> GPHMSSERVLSYAPAFKSFLDTSFFQELSRLKLDVLKLDSTCQPLTVNLDLHNIPKSADQVPLFLTNRSFEKHNNKRTNEVPLQGSIFNFNVLDEFKNLDKQLFLHQRALECWEDGIKDINKCVSFVIISFADLKKYRFYYWLGVPCFQRPSSTVLHVRPEPSLKGLFSKCQKWFDVNYSKWVCILDADDEIVNYDKCIIRKTKVLAIRDTSTMENVPSALTKNFLSVLQYDVPDLIDFKLLIIRQNEGSFALNATFASIDPQSSSSNPDMKVSGWERNVQGKLAPRVVDLSSLLDPLKIADQSVDLNLKLMKWRILPDLNLDIIKNTKVLLLGAGTLGCYVSRALIAWGVRKITFVDNGTVSYSNPVRQALYNFEDCGKPKAELAAASLKRIFPLMDATGVKLSIPMIGHKLVNEEAQHKDFDRLRALIKEHDIIFLLVDSRESRWLPSLLSNIENKTVINAALGFDSYLVMRHGNRDEQSSKQLGCYFCHDVVAPTDSLTDRTLDQMCTVTRPGVAMMASSLAVELMTSLLQTKYSGSETTVLGDIPHQIRGFLHNFSILKLETPAYEHCPACSPKVIEAFTDLGWEFVK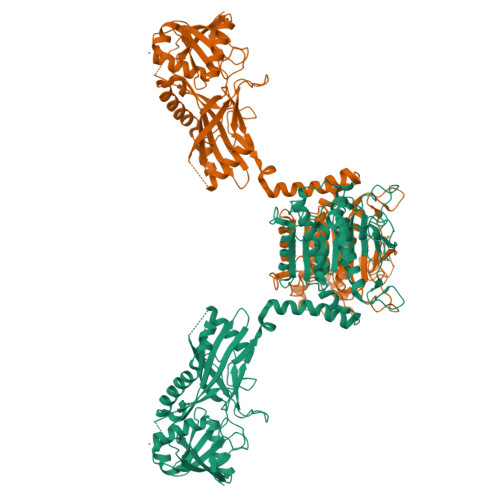KALEHP> GPLGSKL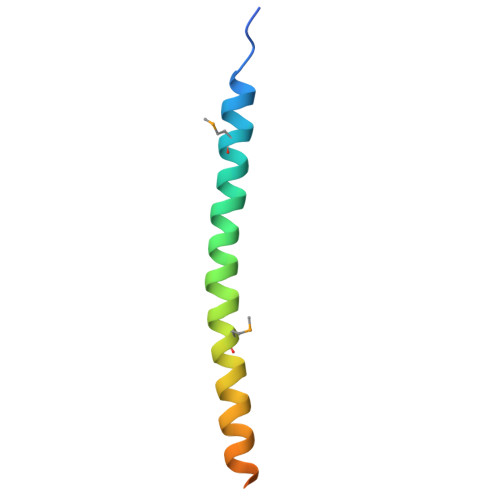PDAAKKMEEAQEALRQAEEERKAKYAKMEAEREAVRQGIRDKYGIKKKEEREAEAQ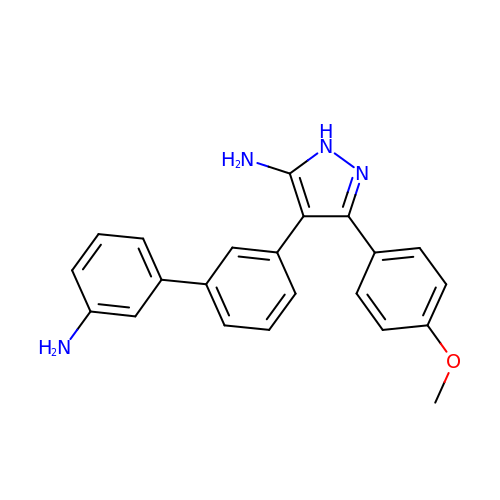4-(3'-amino[1,1'-biphenyl]-3-yl)-3-(4-methoxyphenyl)-1H-pyrazol-5-amine | C22 H20 N4 O | NUTSYDYCFJFYDE-UHFFFAOYSA-N> TGGVQTVTLIPGDGIGPEISAAVMKIFDAAKAPIQWEERNVTAIQGPGGKWMIPSEAKESMDKNKMGLKGPLKTPIAAGHPSMNLLLRKTFDLYANVRPCVSIEGYKTPYTDVNIVTIRENTEGEYSGIEHVIVDGVVQSIKLITEGASKRIAEFAFEYARNNHRSNVTAVHKANIMRMSDGLFLQKCREVAESCKDIKFNEMYLDTVCLNMVQDPSQFDVLVMPNLYGDILSDLCAGLIGGLGVTPSGNIGANGVAIFESVHGTAPDIAGKDMANPTALLLSAVMMLRHMGLFDHAARIEAACFATIKDGKSLTKDLGGNAKC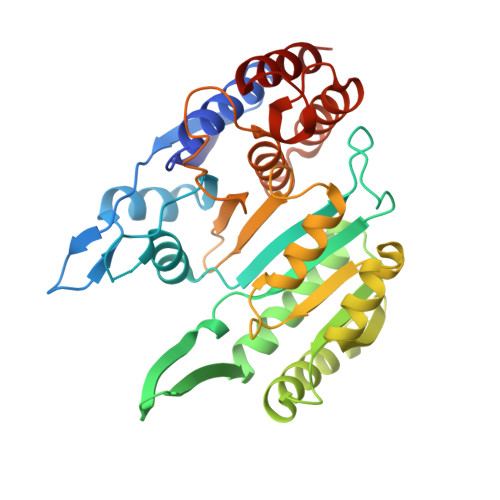SDFTEEICRRVKDLD> KRIVACDDPDFLTSYFAHSRLHHLSAWKANLKDKFLNENIHKYTKITDKDTYIIFHIDFDCFFATVAYLCRSSSFSACDFKRDPIVVCHGTKNSDIASCNYVARSYGIKNGMWVSQAEKMLPNGIKLISLPYTFEQFQLKSEAFYSTLKRLNIFNLILPISIDEAVCVRIIPDNIHNTNTLNARLCEEIRQEIFQGTNGCTVSIGCSDSLVLARLALKMAKPNGYNITFKSNLSEEFWSSFKLDDLPGVGHSTLSRLESTFDSPHSLNDLRKRYTLDALKASVGSKLGMKIHLALQGQDDEESLKILYDPKEVLQRKSLSIDINWGIRFKNITQVDLFIERGCQYLLEKLNEINKTTSQITLKLMRRCKDAPIEPPKYMGMGR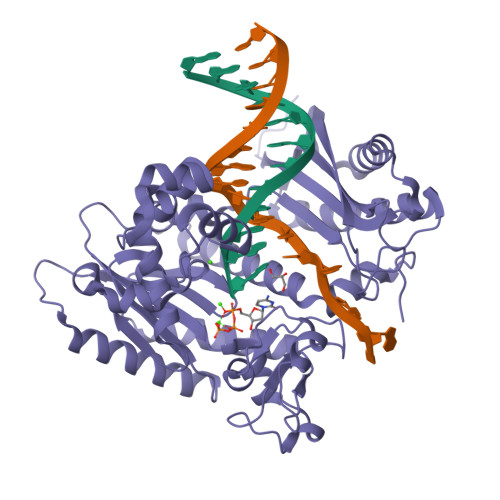CDSFSRSSRLGIPTNEFGIIATEMKSLYRTLGCPPMELRGLALQFNKLVDVGPDNNQLK>[8x]MGFPIPDPYVWDPSFRTFYSIIDDEHKTLFNG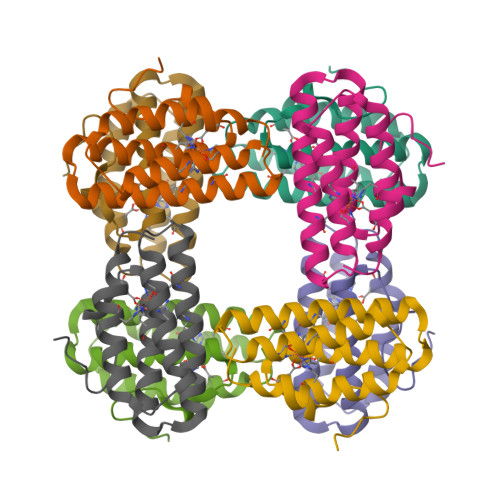IFHLAIDDNADNLGELRRCTGKHFLNEQVLMQASQYQFYDEHKKEHETFIHALDNWKGDVKWAKSWYVNHIKTIDFKYKGKI NuMA is the dynein/dynactin adaptor that in mitosis assists spindle assembly and orientation processes. In metaphase, when spindle positioning takes place, NuMA accumulates at the cortex by association with LGN. The TPR domain of LGN interacting with NuMA comprises 8 tetratricopeptide repeats (TPRs), each consisting of a couple of antiparallel helices organized in a concave super-helical array, in such a way that the first helix-A of each TPR faces the inner side of the super-helix, while the second helix-B is positioned outside. Here, we show that the dynein adaptor NuMA and membrane-localized LGN assemble in oligomers that can form multivalent interactions key to sustain effective pulling on astral MTs.

To gain insights into the topology of the NuMALGNBD:LGNTPR hetero-hexamers, we determined their crystallographic structure at 4.3 Å resolution. Overall, the hetero-hexamers arrange in a donut-shaped architecture, with the backbone of the donut formed by the three LGNTPR protomers concatenated in a head-to-tail fashion, and a central triangular cavity reflecting the threefold symmetry of the assembly. In such an arrangement, the flexible NuMA chains thread in-between two adjacent LGN subunits, and then line in the internal groove of the TPR domain. The donut assembly is promoted primarily by the formation of a four-helix bundle containing the TPR8 and the capping helix of one LGNTPR protomer (named here LGN-1 for clarity), and the N-terminal helix preceding the TPR1 of the neighboring LGNTPR molecule (LGN-2), in a sort of molecular grip. This topology explains why deletion of residues 7–13 or 350–367 of LGNTPR impairs hexamer formation. More specifically, residues 1864–1880 of NuMA-1 start with two helical turns interrupted at Pro1874, where the chain bends in an elongated polypeptide, and packs against helices-A/B of the second TPR motif of the LGN-2 subunit, facing Leu54LGN-2 and Tyr58LGN-2. Analytical SEC experiments revealed that disrupting the NuMA1861–1880:LGNTPR interface prevents hexamer formation, confirming that hooking of NuMA1861–1880 on LGNTPR is essential for oligomerization. We conclude that NuMA has a bipartite LGN-binding domain consisting of a nanomolar affinity peptide spanning residues 1900–1928 and a disjunct upstream oligomerizing motif encompassing aa 1861–1880, which is essential for hetero-hexamer formation. The toroidal architecture of the hexamers is allowed by the characteristic TPR array of LGN featuring a long TPR4 that confers a pronounced curvature to the scaffold.

>[12x]GPLGSMFHVRYRMEASCLELALEGERLCKSGDCRAGVSFFEAAVQVGTEDLKTLSAIYSQLGNAYFYLHDYAKALEYHHHDLTLARTIGDQLGEAKASGNLGNTLKVLGNFDEAIVCCQRHLDISRELNDKVGEARALYNLGNVYHAKGKSFGCPGPQDVGEFPEEVRDALQAAVDFYEENLSLVTALGDRAAQGRAFGNLGNTHYLLGNFRDAVIAHEQRLLIAKEFGDKAAERRAYSNLGNAYIFLGEFETASEYYKKTLLLARQLKDRAVEAQSCYSLGNTYTLLQDYEKAIDYHLKHLAIAQELNDRIGEGRACWSLGNAYTALGNHDQAMHFAEKHLEISREVGDKSGELTARLNLSDLQMV;>GPLGSPDYGNSALLSLPGYRPTTRSSARRSQAGVSSGAPPGRNSFYMGTCQDEPEQLDDWNRIAELQQRNR[12x]>[4x]GPHMMSGEKRVLSGRVAVVTGSRKGIGLGIAMRLAMAGADVVLNGFRQSPEDSAIVEKVAAYGTRVRCFAANMKDRAQVEALIKFTEKELGAVEILVNNAGIQHVSPVETFPSDKWDEIIALNLT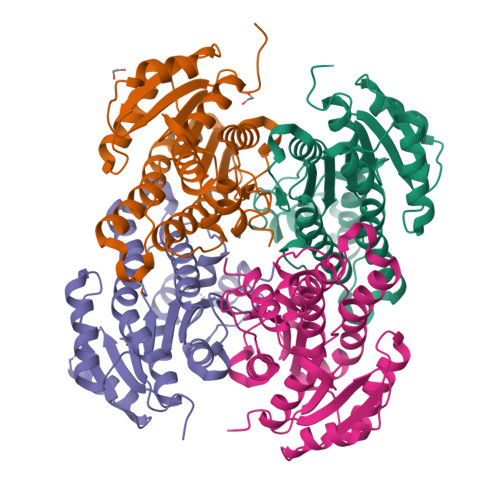SAFHATQLCLPSMRQRGWGRIINIASVQGLVGSMNKSAYCAAKHGLIGFTKVVALETATTGITCNAICPGYVYTPLVEEQIKAVAEAKYGGDMEAATQAFLCEKQPAKAFVTVEQVGDAAVFLASPGADMIRGTTITVDGGWVAQ(S)-Tioconazole | C16 H13 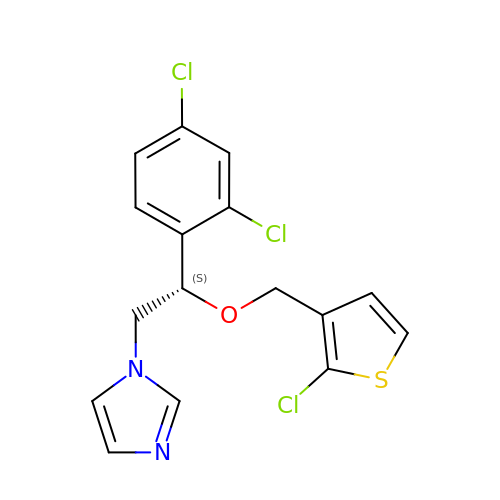Cl3 N2 O S | QXHHHPZILQDDPS-OAHLLOKOSA-N> MEAVLSRQAATAEAIGRFQDSSTSVGLVAGSPSTRIRRQADNVVLKSTSQAGDTLNDVIQDPTRRNKLINDNNLLKGIIMGRDGPVPSSRELIVRPDTLRAIINNRATIETTTMEAEFTETLMESNYNSASVKVSAPFITANSEYSESSSFKNTETEKSMYTSSRYLFPQGRIDFTTPDSGFDDVIKLSPQFTSGVQAALAKATGTEKREALQNLFQEYGHVFRTKVHIGGVLSAHTMETFSRSENETEVKQDVKAGLEGAVKGWGGGATAGHGNTQGTITTSQNRKLNVKYIVNGGDYTKIQNTEEWVASTNQSEH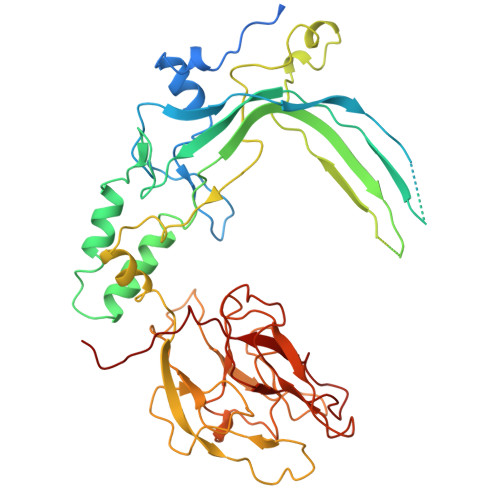WRVIEVTEVTAVADLLPQPIRGQVKDLLKPLLGKWVDVEKVPGLESLPVSVYRPKGAIPAGWFWLGDTADASKALLVKPTLPARSGRNPALTSLHQGSGMTEQPFVDLPQYQYLSTYFGSFAHDTPPGSTLRGLRPDHVLPGRYEMHGDTISTAVYVTRPVDVPFPEDECFDLKSLVRVKLPGSGNPPKPRSALKKSMVLFDSGEK> APSVKGVSFDQANNLLIEPARIEEEELTLTILRQTGGLGISIAGGKGSTPYKGDDEGIFISRVSEEGPAARAGV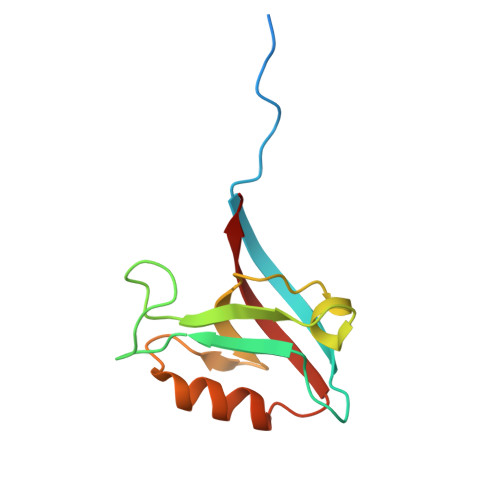RVGDKLLEVNGVALQGAEHHEAVEALRGAGTAVQMRVWRERM>[4x]MPLTEIQVESYKKALQADVPPEKRENVGIQAAFKETFPIEEGDKGKGGLVLDFLEYRIGDPPFSQDECREKDLTYQAPLYARLQLIHKDTGLIKEDEVFLGHLPLMTEDGSFIINGADRVIVSQGGRTVGELMADQFRVGLARLARGVRERMVMGSPDTLTPAKLVNSRPLEAALREFFSRS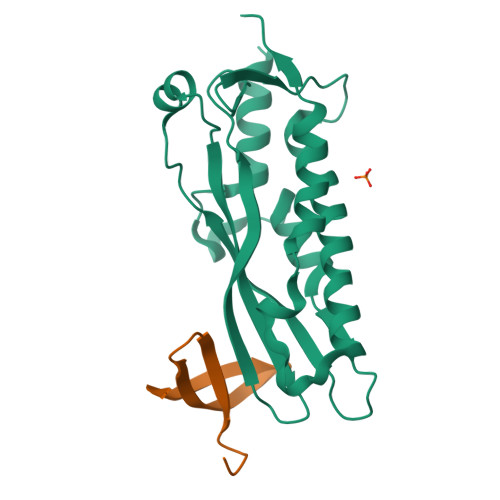QLSQFK;>GPHMPGDYLIHPEHGVGQYLGLETREVLGVKRDYLVLRYKGEGKLYLPVEQLPLLKRHPGTTDDPPELSSL[4x]>XGEIAQAIKEIAKAIKE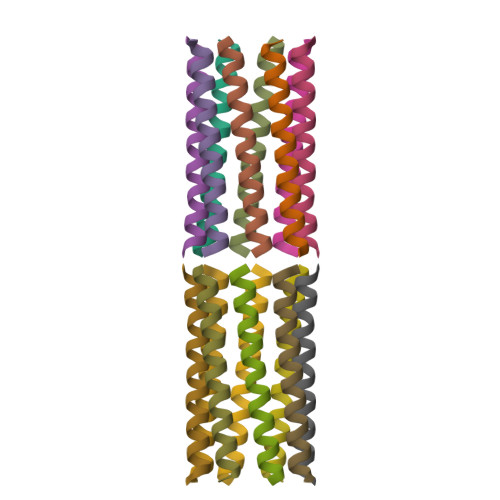VAWAFKEIAQAIKGX[2x]Quantitative data about starch phosphorylase protein abundance and enzyme activity are lacking and no crystal structure of a plastidic plant starch phosphorylase has been reported so far. It is known that starch phosphorylases are members of the CAZy GT35 family of glycosyltransferases and catalyze the reversible transfer of glucosyl residues from a glucose donor onto the non-reducing end of an α-glucan chain. While Pho2 is localized in the cytosolic compartment, Pho1 is a true starch phosphorylase that acts on starch in the plastids of the plant cell. We determined the crystal structures of HvPho1, the first crystal structure of a plastidic plant starch phosphorylase. A native structure of HvPho1 and two complexes with acarbose and maltotetraose were solved and refined to resolutions of 2.7 Å, 2.9 Å and 3.0 Å respectively.

The native structure was obtained from a crystal formed from a drop in the absence of substrates, which was then mixed with another drop, to which 10 mM maltoheptaose had been added. The intention had been to obtain a crystal of the complex, but no maltooligosaccharide ligands were observed in the electron density. TLC analysis of a similar crystal-drop, where HvPho1 was co-crystallized with maltoheptaose, revealed that the maltoheptaose was hydrolyzed, mostly to maltose and maltotriose. Accordingly no maltooligosaccharides were observed in the electron density of this HvPho1 crystal and we refer to it simply as the “native” crystal. Two almost identical HvPho1 monomers (R.M.S.D. = 0.19 Å), related by a quasi-crystallographic translation, are present in the asymmetric unit of the crystal. One of them had weak electron density for a citrate anion in the active site, likely a crystallization artifact as citrate was part of the mother liquor. Consequently, one citrate molecule was included in the final model. The structure is similar to those of the cytosolic phosphorylase of A. thaliana (AtPHS2), rabbit muscle phosphorylase B and E. coli MalP, including the presence of a pyridoxal-5’-phosphate prosthetic group covalently bound to Lys814 and similar dimerization interfaces. An overlay on rabbit muscle glycogen phosphorylase b suggests that HvPho1 does not contain a functional polysaccharide storage site. The ordered part of the L78 insertion overlaps with the location where glycogen (or starch) binds to phosphorylase, in a position incompatible with maltooligosaccharide binding.

>MRSVASDREVRGPASTEEELSAVLTSIDSSAIASNIQHHADFTPLFSPEHSSPLKAYHATAKSVFDSLIMNWNATYDYYNKVNAKQAYYLSMEFLQGRALTNAIGNLELTGQYAEALKQLGHNLEDVASQEPDPALGNGGLGRLASCFLDSLATLNYPAWGYGLRYRYGLFKQIITKDGQEEVAENWLEMGNPWEIVRNDVSYPVKFYGKVVEGTDGRKHWIGGENIKAVAHDVPIPGYKTKTTNNLRLWSTTVPSQNFDLGAFNAGDHAKANEAHLNAEKICHVLYPGDESSEGKILRLKQQYTLCSASLQDIISRFESRAGDSLNWEDFPSKVAVQMNDTHPTLCIPELMRILMDIKGLSWNEAWSITERTVAYTNHTVLPEALEKWSLDIMQKLLPRHVEIIETIDEELMNNIVSKYGTADISLLKQKLKDMRILDNVDLPASVAKLFIKPKEKRGKLLVESLESIAEADEKTESQEVENILSETTEKKAESDSEEAPDAEKEDPEYELDPFAKYDPQFPRVVRMANLCVVGGHSVNGVAEIHSEIVKQDVFNSFYEMWPTKFQNKTNGVTPRRWIRFCNPELSTIISKWIGSDDWILNTDKLAGLKKFADDEDLQSEWRTAKRNNKMKVVSLIRDKTGYIVSPDAMFDVQVKRIHEYKRQLLNILGIVYRYKKMKEMSAKDRRKSFVPRVCIFGGKAFATYVQAKRIVKFITDVAATVNYDPDIGDLLKVVFVPDYNVSVAETLIPASELSQHISTAGMEASGTSNMKFAMNGCLLIGTLDGANVEIREEVGEENFFLFGAHAPEIAGLRQERAEGKFVPDLRFEEVKEYVRSGVFGTSNYDELMGSLEGNEGYGRADYFLVGKDFPSYIECQEKVDEAYRDQKLWTRMSILNTAGSPKFSSDRTIHEYAKDIWDISPVIMPTFPDIENLYFQG[2x]>MDIGIN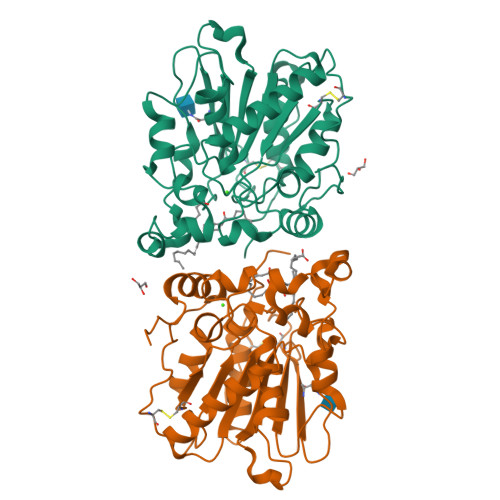SDPNSATVASDPVGPEQISFLPAKLYSSLAPTALPPGTNDWTCQPSAAHPRPVVLVHGTWANRYDSFAMIAPHLKRAGYCVYALNYGDENVSVLGQLPGLYATQTIKPAGGEISSFVDQVLDSTGADQVDMFGWSQGGIAARSYLKFYGGTNAANPAANKVKNLITFGATNHGTTLSGLGALAGQLAPATIPPVLGPAAADQLIDSPFLTELNAGGDTQPGVTYTIIGSRYDEVSTPYQRTFLTAGPGATVNNITLQNGCEIDLSDHLSGLYSYRLVGLVKKALDPTGNVYVPCLPNAPVLEHHHHHH[4x]>CGGAGGAACUACUGUCUUCACGCC[2x];>GCGUGUCGUGCAGCCUCCGG[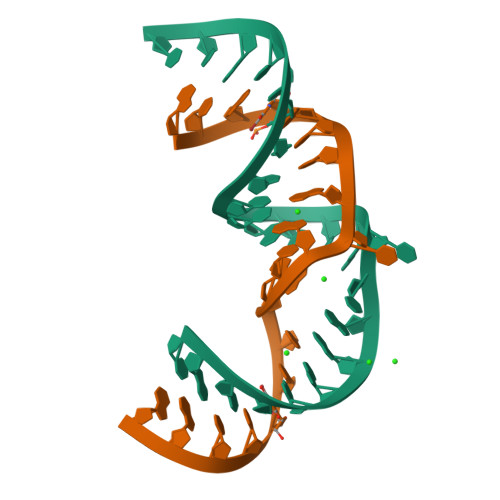2x]4-phenoxybenzoic 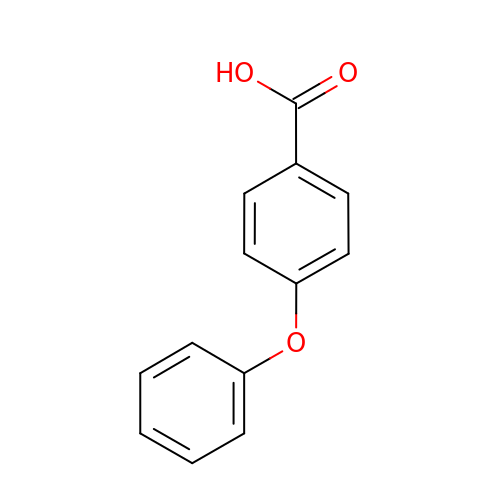acid | C13 H10 O3 | RYAQFHLUEMJOMF-UHFFFAOYSA-N> MAKKTSSKGKLPPGPTPFPIIGNILQIDAKDISKSLTKFSECYGPVFTVYLGMKPTVVLHGYEAVKEALVDLGEEFAGRGSVPILEKVSKGLGIAFSNAKTWKEMRRFSLMTLRNFGMGKRSIEDRIQEEARCLVEELRKTNASPCDPTFILGCAPCNVICSVIFHNRFDYKDEEFLKLMESLHENVELL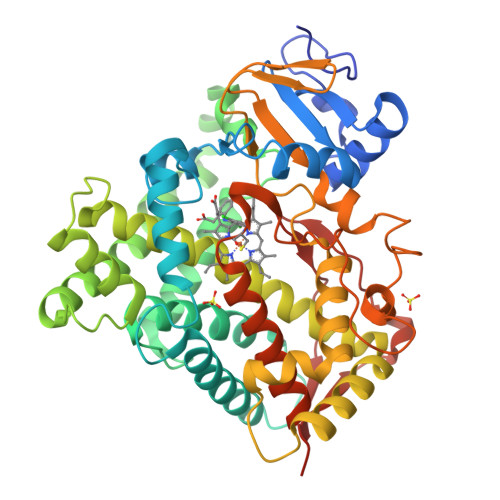GTPWLQVYNNFPALLDYFPGIHKTLLKNADYIKNFIMEKVKEHQKLLDVNNPRDFIDCFLIKMEQENNLEFTLESLVIAVSDLFGAGTETTSTTLRYSLLLLLKHPEVAARVQEEIERVIGRHRSPCMQDRSRMPYTDAVIHEIQRFIDLLPTNLPHAVTRDVRFRNYFIPKGTDIITSLTSVLHDEKAFPNPKVFDPGHFLDESGNFKKSDYFMPFSAGKRMCVGEGLARMELFLFLTSILQNFKLQSLVEPKDLDITAVVNGFVSVPPSYQLCFIPIHHHH> MSPVGRLFLGSKLPAQTWQSFRLQPALPQFAQKRFFSGGAAKPSWHVAREHRFGPTLPDHAYYGEHATYNYFVLFIRGMRPYLEKIFGDCASTIKNAAVAVYRPVNAFVVKHNPDLRLQFVAFASFIATHMAITKEFNDMYQRLVDITSLLELQAAQLHAS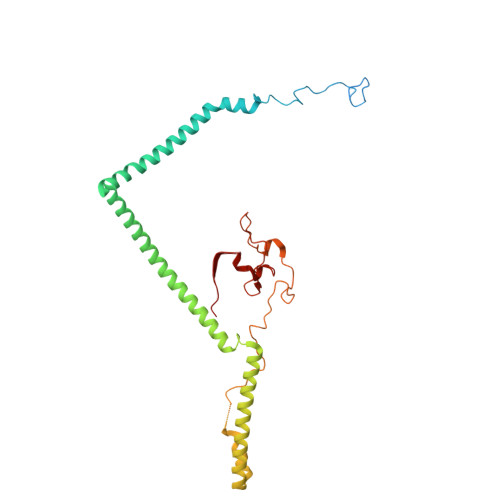EGFWDSESEQQEARLQRHAEHRNDLETTWEEALREATLARNFDVLVSYLNHGTSDGCGEHGACGHSGQNGIPPSVTWNFNAMPYGKENPDTKTFPIPDHEQPYRAFSLGFTANNLSGNWGDYIDRQDNKNALMRPARMMFTDVFIPTTK> SGRGEAETRECIYYNANWELE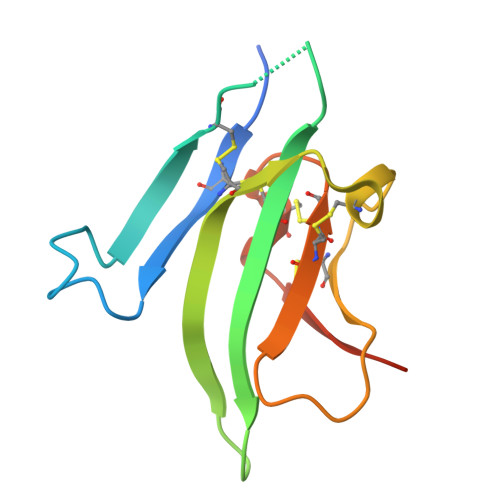RTNQSGLERCEGEQDKRLHCYASWRNSSGTIELVKKGCWLDDFNCYDRQECVATEENPQVYFCCCEGNFCNERFTHLPEPLVPR> MGRKKIQIQRITDERNRQVTFTKRKFGLMKKAYELSVLCDCEIALIIFNHSNKLFQYASTDMDKVLLKYTEYNEPHESRTNADIIE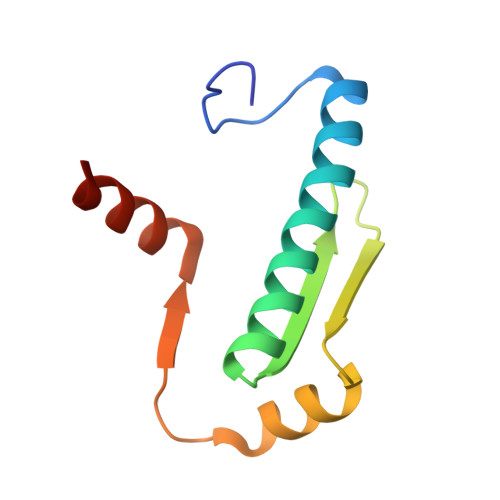TLRKKGFNG>MAHHHHHHSSGLEVLFQGPMTHSVVELIEIESAIIQVKMQDRTHKNAFSQELTDDLIQAFEYIRQNPKYKAVILTGYDNYFASGGTQEGLLRIQQGLTKFTDDNLYSLALDCEIPVIAAMQGHGIGGGFVMGLFADIVILSRESVYTANFMKYGFTPGMGATFIVPKKLGFSLAQEILLNAGSYRGADLEKRGVPFKVLPRAEVLDYAVELAQELAEKPRNSLVTLKDHLVAPLRDQLPRVIEQELMMHEATFHHEEVKSRIKGLYGN[3x]

In this study we present a structural and functional description of the bacillaene synthase β-branching enzymes PksH and PksI. These biocatalysts are responsible for the final two steps in β-methyl branch incorporation in this PKS/NRPS pathway. There is a single active site per PksI monomer, with each active site positioned on the periphery of the trimer, ~ 43 Å from one other. Akin to PksH, PksI adopts a characteristic CS fold, with a ββα core, that comprises two approximately perpendicular -sheets surrounded by -helices.

Assays were conducted using WT PksI, along with the point mutants PksI-H230A, PksI-H235A, PksI-K80A, PksI-K232A. Of the four PksI mutants investigated only PksI-H230A was found to be catalytically compromised, with barely detectable activity for 3-methyl glutaconyl-SNAC and significantly impaired activity for 3-methyl glutaconyl-CoA. Surprisingly, PksI-K80A and PksI-K232A both display catalytic activities akin to that of WT-PksI, with no evidence of functional impairment. In tandem with kinetic assays, the crystal structures of PksI-K80A, PksI-K232A and H230A were determined. The active sites of each of these enzymes displays the ground state “closed” conformation as observed in the WT enzyme, with no evidence of significant structural perturbations within the active site. These data thus imply that the observed kinetic effects are not attributable to global or local structural reorganization within the enzyme as a consequence of the amino acid substitutions made. Crystal structures of the mutants PksI_K80A, PksI K232A and PksI H230A revealed no significant changes in active site architecture beyond side chain identity. We thus propose a His230 dependent mechanism wherein this residue has a dual function both catalyzing decarboxylation and to act as a proton donor to the decarboxylated intermediate 7 to give the reaction product.NAMPT functions as a homo-dimeric enzyme that catalyzes the rate limiting step in the primary salvage pathway for NAD synthesis, the transfer of a phosphoribosyl residue from 5-phosphoribosyl-1-pyrophosphate (PRPP) to nicotinamide (NAM) to produce nicotinamide mononucleotide (NMN). Crystal structures of NAMPT in numerous ligand-bound forms have been reported. These structures consistently display a NAMPT homo-dimer with two essentially identical active sites at the dimer interface. Typical NAMPT inhibitors were found to occupy the portion of active site responsible for NAM binding and a tunnel-shaped cavity extending from the NAM binding site. Furthermore, we determine the crystal structures of six NAMPT mutants in the apo form and in complex with various inhibitors and present a definitive model to explain the differential effects of the mutations on various structural classes of NAMPT inhibitors.

The crystal structures of NAMPT S165F/Y revealed a somewhat surprising conformational change in a small helical structural motif spans the sequence G383GGLLQ388. We designate this motif as “380GRS” to reflect its position in the primary sequence, and its glycine rich characteristic. As the structural consequences of S165F and S165Y are essentially identical, we focus on the S165F structure in the following discussion. A helical structure of 380GRS is crucial for PRPP binding, as it is situated in the PRPP binding site and the electric dipole moment developed in the helix can complement the negative charges associated with the PRPP 5′-phosphate group. The unwinding of the 380GRS in S165 mutants rendered the structure less compatible with the binding of PRPP. Our structural studies thus reveal that the S165 mutation modulates NAMPT activity by interfering with PRPP binding in an allosteric manner. Consistent with the structural observations, S165F/Y mutant NAMPT proteins required approximately 500 fold more PRPP compared to the wild-type protein and the other NAMPT mutants. Structural analyses of S165 NAMPT mutant proteins establish the critical role of the 380GRS in NAMPT catalysis. Crystal structures revealed a previously underappreciated conformational flexibility in this secondary structure element that can be exploited by resistance mutations through an allosteric mechanism.

>[2x]MNPAAEAEFNILLATDSYKVTHYKQYPPNTSKVYSYFECREKKTENSKLRKVKYEETVFYGLQYILNKYLKGKVVTKEKIQEAKDVYKEHFQDDVFNEKGWNYILEKYDGHLPIEIKAVPEGFVIPRGNVLFTVENTDPECYWLTNWIETILVQSWYPITVATNFREQKKILAKYLLETSGNLDGLEYKLHDFGYRGVSSQETAGIGASAHLVNFKGTDTVAGLALIKKYYGTKDPVPGYSVPAAEHSTITAWGKDHEKDAFEHIVTQFSSVPVSVVSDSYDIYNACEKIWGEDLRHLIVSRSTQAPLIIRPDSGNPLDTVLKVLEILGKKFPVTENSKGYKLLPPYLRVIQGDGVDINTLQEIVEGMKQKMWSIENIAFGSGGGLLQKLTRDLLNCSFKCSYVVTNGLGINVFKDPVADPNKRSKKGRLSLHRTPAGNFVTLEEGKGDLEEYGQDLLHTVFKNGKVTKSYSFDEIRKNAQLNIELEAAHHLEHHHHHHHH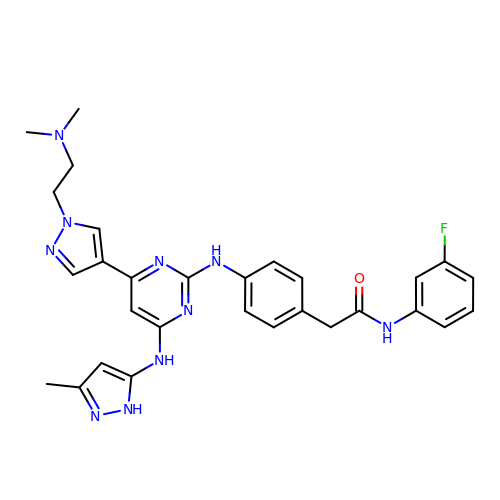2-[4-[[4-[1-[2-(dimethylamino)ethyl]pyrazol-4-yl]-6-[(3-methyl-1~{H}-pyrazol-5-yl)amino]pyrimidin-2-yl]amino]phenyl]-~{N}-(3-fluorophenyl)ethanamide | C29 H31 F N10 O | PVCJCKVFTUXUMC-UHFFFAOYSA-N Pendrin (SLC26A4) is an anion exchanger that mediates bicarbonate (HCO3−) exchange for chloride (Cl−) and is crucial for maintaining pH and salt homeostasis in the kidney, lung, and cochlea. Pendrin also exports iodide (I−) in the thyroid gland. Pendrin mutations in humans lead to Pendred syndrome, causing hearing loss and goiter. Here, we present structures of pendrin from Sus scrofa (ssPendrin), which is 90% identical to human pendrin, in complex with either I−, HCO3−, or Cl−; ssPendrin in the apo-state; and ssPendrin in the presence of NFA, which inhibits anion transport.

The structures of ssPendrin in the presence of I−, HCO3− or Cl− were determined by cryo-electron microscopy (cryo-EM) to an overall resolution of 2.8 Å, 2.7 Å, and 2.5 Å, respectively. The densities at the S1 and S2 sites are at ~5σ level in both the Cl−- and HCO3−-bound ssPendrin structures, and the densities are at ~13 σ in the I−-bound structure. The overall position and coordination of the two anions are almost identical in all three structures, with subtle adjustments of coordinating atoms. To functionally corroborate our structural observation of two anion binding sites, we performed 125I− saturation binding by using the scintillation proximity assay (SPA). Nonlinear regression fitting of the data was performed to obtain the EC50, the Hill coefficient, and molar ratios of I−-to-ssPendrin binding, revealing that one molecule of ssPendrin-WT can simultaneously bind two I− with an EC50 of ~10 mM, and a Hill coefficient of ~2. In contrast, both tested ssPendrin mutants with either impaired S1 or S2 anion binding site exhibited a molar binding stoichiometry of ~1. Whereas the EC50 for both mutants were comparable to that of the WT, the Hill coefficients for both mutant variants were reduced to ~1, indicative of the loss of allosteric binding between the two identified anion sites. Saturation binding studies using 125I− support that pendrin under equilibrium conditions can bind two anions (e.g., I−) simultaneously. In all three ssPendrin structures, the anion binding sites are solvent accessible from the intracellular side through a large cavity formed between the transport and scaffold domains. Thus, the structures of ssPendrin are captured in the inward-facing conformation.

>[2x]MAAPGSRLEPPPLPEYSCSYVVSRPVYSELAFQQQYERRLQERKTLRESLAKRCSCSRKRTLGVLKTLLPVLDWLPKYRIKEWLLSDIISGVSTGLVGTLQGMAYALLAAVPVGYGLYSAFFPILTYFIFGTSRHISVGPFPVVSLMVGSVVLSMAPDEHFIISSSNGTALNTTVIDFAARDAARVLIASTLTLLVGIIQLIFGGLQIGFIVRYLADPLVGGFTTAAAFQVLVSQLKIVLNVSTKNYNGILSIIYTLIEIFQNIGNTNLADFIAGLLTIIICMAVKELNDRFKHKIPVPIPIEVIVTIIATAISYAVNLEKNYNAGIVKSIPRGFLPPEIPPISLFSEMLTASFSIAVVAYAIAVSVGKVYAIKYDYTIDGNQEFIAFGISNIFSGFFSCFVATTALSRTAVQESTGGKTQIAGIISAAVVMIAIVALGKLLEPLQKSVLAAVVIANLKGMFMQVCDVPRLWRQNKTDAVIWVFTCIASIILGLDLGLLAGLMFGFLTVVVRVQFPSWNSLGSIPNTDIYRSTKDYKNIEEPEGVKILRFSSPIFYGNVDGLKKCIKSTVGFDAIRVYNKRLKALRKIQKLIKKGQLRATKNGIISDAGSSNNAFEPDEDIEDPEELDIPTKEIEIQVDWNSELPVKVNVPKVPIHSLVLDCGAVSFLDVVGVRSLRMIVKEFQRIDVHVYFASLQDHVIEKLEQCGFFNDSIRKDIFFLTVHDAILHLRSQVKSQEVQDSILETITLIQDCKDPLELMEAELIEEELDVQDEAMRRLAS>[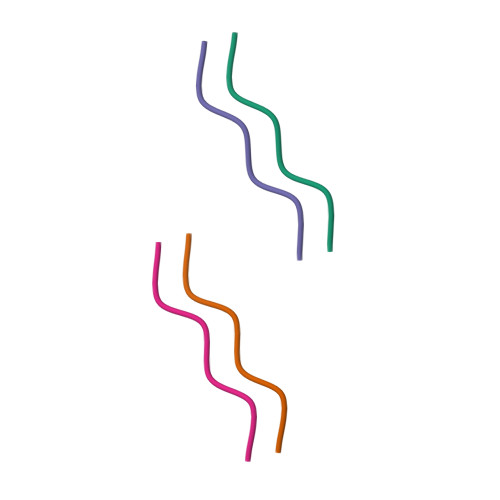2x]VQIVYK5-[4-(DIMETHYLAMINO)PHENYL]-6-[(6-MORPHOLIN-4-YLPYRIDIN-3-YL)ETHYNYL]PYRIMIDIN-4-AMINE 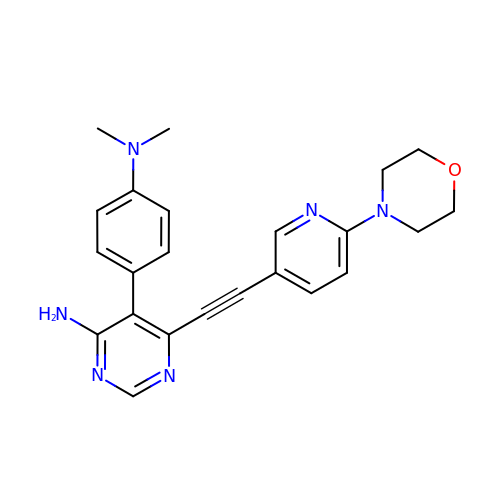| C23 H24 N6 O | AINVOEOJEKKMKB-UHFFFAOYSA-N>NTKYNKEFLLYLAGFVDGDGSIIAQIKPNQSYKFKHQ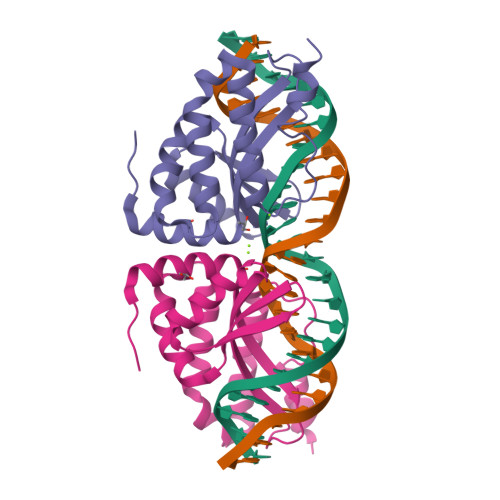LSLTFQVTQKTQRRWFLDKLVDEIGVGYVRDRGSVSNYILSEIKPLHNFLTQLQPFLKLKQKQANLVLKIIEQLPSAKESPDKFLEVCTWVDQIAALNDSKTRKTTSETVRAVLDAA[2x]>MDKFRVQGPTRLQGEVTISGAKNAALPILFAALLAEEPVEIQNVPKLKDIDTTMKLLTQLGTKVERDGSVWIDASNVNNFSAPYDLVKTMRASIWALGPLVARFGQGQVSLPGGCAIGARPVDLHIFGLEKLGAEIKLEEGYVKASVNGRLKGAHIVMDKVSVGATVTIMSAATLAEGTTIIENAAREPEIVDTANFLVALGAKISGQGTDRITIEG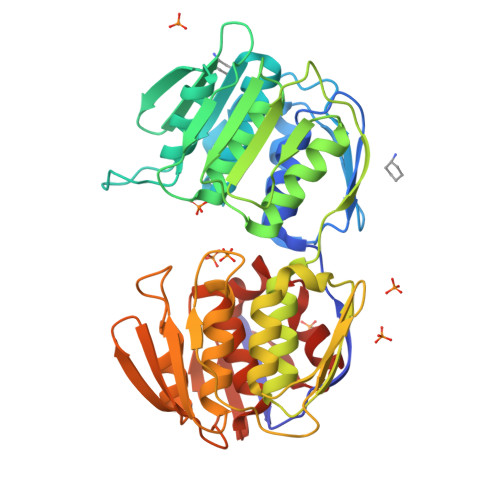VERLGGGVYRVLPDRIETGTFLVAAAISGGKIVCRNAQPDTLDAVLAKLREAGADIETGEDWISLDMHGKRPKAVTVRTAPHPAFPTDMQAQFTLLNLVAEGTGVITETIFENRFMHVPELIRMGAHAEIESNTVICHGVEKLSGAQVMATDLRASASLVLAGCIAEGTTVVDRIYHIDRGYERIEDKLRALGANIERVKGE[2x]> NSNNKRAP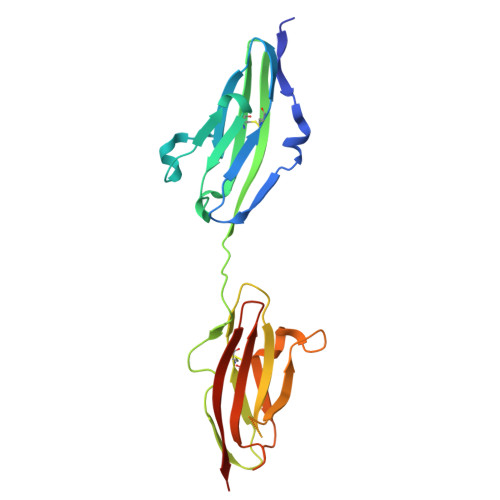YWTNTEKMEKRLHAVPAANTVKFRCPAGGNPMPTMRWLKNGKEFKQEHRIGGYKVRNQHWSLIMESVVPSDKGNYTCVVENEYGSINHTYHLDVVERWPHRPILQAGLPANASTVVGGDVEFVCKVYSDAQPHIQWIKHVEKNGSKYGPDGLPYLKVLKAAGVNTTDKEIEVLYIRNVTFEDAGEYTCLAGNSIGISFHSAWLTVLPAPGRE>GKHILVASVKEVYSKVDQLKAGDTLLLKDGIYKDIQLVVKRSGSKEKPIVIAAQNGGKVFFTGDAKVELRGEYLVLKDIYFKDGNRNVNQWKSHGPGLVAIYGSYNRVTGCVFNAFDEANSAYITTSLTEEGKVPKHCRIDHCVFTDKITFDQVINLNNRPRADKESKVLGEAMYHRIDHCFFSNPPKPGNAGGGIRVGYYRNDIGRCLIDSNLFVRQDSEAEIVTSKSQENVYYGNTILNCQGTLNFRHGDKQVALNNFFISTDNKYGYGGMFVWGSQHIIANNYFNLKKTIKARGNAALYLNPGPEGSEHALAFNSLIVNNFFDDNNGYDINFEPLLERRKEFAKEVNAEFKLPYNITIEGNLFASKQGDKHIPFLGNLDKNNLQNNYSFGQMANDKLFTNVKPTTDGSYNPQSYKGYQLANVKDIKNIEGIDLDIQNLINKGIE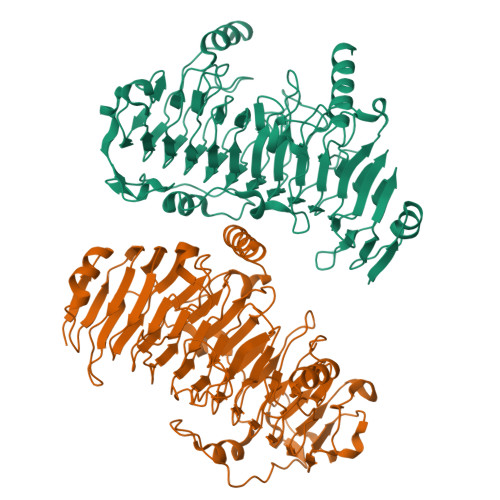GNPLTWNDVRPSWLVEIPGSYAKEGTLDQETKIRFQRVLARDRNN[2x]> SNIQTGAERMPHDLSHLGFLAGQIGRLITISTTPVIAGDSFEMDAVGALRLSPLRRGLAIDSTVDIFTFYVPHRHVYGEQWIKFMKDGVNATPLPTVNTTGYIDHAAFLGTINPDTNKIPKHLFQGYLNIYNNYFKAPWMPDRTEANPNELNQDDARYGFRCCHLKNIWT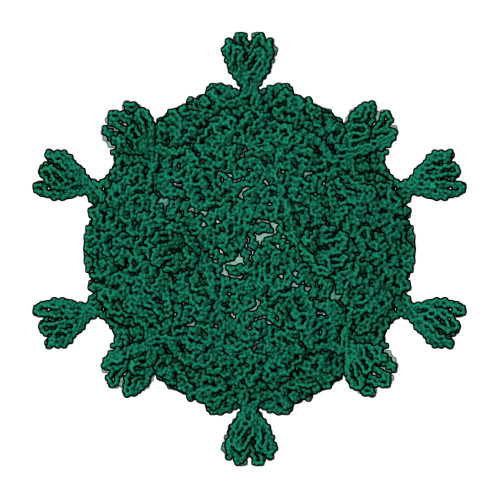APLPPETELSRQMTTSTGMAPVTTKFRDVPNLSGTPLIFRDNKGRTIKTGQLGIGPVDAGFLVAQNTAQAANGERAIPSNLWADLSNATSIDIMGLQAAYANLHTDQERDYFMQRYRDVISSFGGKTSYDADNRPLLVMRSNLWASGYDVDGTDQTSLGQFSGRVQQTYKHSVPRFFVPEHGTMFTLALVRFPPTATKEIQYLNAKGALTYTDIAGDPVLYGNLPPREISMKDVFRSGDSSKKFKIAEGQWYRYAPSYVSPAYHLLEGFPFIQEPPSGDLQERVLIRHHDYDQCFQSVQLLQWNSQVKFNVTVYRNLPTTRDSIMTS Inherited missense mutations in the myocilin (MYOC) gene, within its olfactomedin (OLF) domain, constitute the strongest genetic link to primary open-angle glaucoma via a toxic gain of function, and thus MYOC is an attractive precision-medicine target. Myocilin has no known function, and there is no glaucoma phenotype in Myoc knockout mice or in individuals with a homozygous N-terminal truncation mutation or hemizygous deletion of MYOC, but rare non-synonymous coding mutations lead to toxic intracellular sequestration of misfolded myocilin. However, not all mutations in MYOC cause glaucoma, and common variants are expected to be neutral polymorphisms. Among the common features associated with pathogenic myocilin misfolding, we demonstrate that a single metric, OLF thermal stability, can robustly segregate benign from early-onset disease variants.

Overall, nine variants (T256M, R296H, L303I, S313F, V329M, S331L, E352K, A427T, and V499I) were considered likely to be benign. Assessment of spent media from cells expressing each of the 16 full-length myocilin variants revealed WT-like secretion for T256M, R296H, L303I, S313F, V329M, S331L, T353I, A445V, V449I and K500R. Structural integrity was further confirmed by high-resolution crystal structures, which were solved for 11 OLF variants. No gross changes from WT OLF were detected for the structures of T293K, R296H, L303I, V329M, S331L, E352K, T353I, K398R, A445V, V449I or K500R, indicating that these mutations are accommodated within the native five-bladed β-propeller fold and do not perturb the dinuclear calcium-containing site. In addition to the five variants that we predicted initially to be benign (T293K, T353I, K398R, A445V and K500R), our study reveals seven more (T256M, R296H, L303I, V329M, S331L, E352K and V499I) that are indistinguishable from WT OLF across multiple assays. Thus, our data indicate these should also be considered benign.

> LKESPSGYLRSGEGDTGCGELVWVGEPLTLRTAETITGKYGVWMRDPKPTYPYTQETTWRIDTVGTDVRQVFEYDLISQFMQGYPSKVHILPRPLESTGAVVYLGSLYFQGAESRTVIRYELNTETVKAEKEIPGAGYHGQFPYSWGGYTDIDLAVDEAGLWVIYSTDEAKGAIVLSKLNPENLELEQTWETNIRKQSVANAFIICGTLYTVSSYTSADATVNFAYDTGTGISKTLTIPFKNRYKYSSMIDYNPLEKKLFAWDNLNMVTYDIKLSKM Proliferating Cell Nuclear Antigen (PCNA) is a member of the sliding clamp family of DNA-replication accessory proteins. In most organisms PCNA is a homotrimer, in which its three subunits adopt a doughnut-shaped structure in a head-to-tail arrangement; this toroidal structure is extremely conserved in protozoa, humans, yeast and plants. The structure of PCNA is comprised by two α+β domains joined by an inter-domain connecting loop (IDCL). The inner face of the toroid has an array of basic residues positioned to provide favorable electrostatic interactions with the DNA-phosphate backbone.

Herein we report the x-ray structure analysis of the first crustacean recombinant PCNA (LvPCNA) and a model where PCNA interacts with viral DNA polymerase PIP-box as an approach toward structural understanding this feasible interaction. LvPCNA eluted in a complex of approximately 90 kDa, indicating that this protein assembles as a trimer in solution. Accordingly to this previous result the molecular replacement found a trimer in the asymmetric unit. LvPCNA had the cognate fold comprised by β-α-β5-α-β-β-β-IDCL-β-α-β5-α-β-β-β topology with pseudo symmetry within each monomer. The backbone cartoon shows the canonical structure and although the IDCL (residues 117–133) had poor electron density, the density was conclusive to include the coordinates of those residues in the final model. LvPCNA amino acid sequence is highly conserved among species and is structurally similar when compared with Drosophila PCNA, as it had a root mean square deviation (RSMD) of 0.5 Å for the α-carbon backbone. The central hole is highly positive charged as shown in Figure 3 and has a diameter of 30.5 Å, large enough to accommodate the double helical DNA and slide freely on it. A peptide sequence containing the WSSV DNA polymerase PIP box was modeled and docked into the crystallographic structure of shrimp PCNA, which is its natural host. However, this is a tight packing cavity as obtained by docking, where mostly hydrophobic interactions are leading the binding, the hydrophobic cavity is represented in a surface image where the PIP-box peptide is positioned and drawn as sticks. This pocket comes mainly from the IDCL (G127, P129, T131), central loop (S43, H44, V45, L47) and from C-terminus (F250, L251, A252, P253, I255) residues. The results from docking suggest that WSSV polymerase has the capacity of binding the LvPCNA in the same way that most PCNA binding proteins do.

>[3x]MFEARLVQGSLLKKVLEAIKDLLNEASWDCADSGIQLQAMDNSHVSLVSLNLRAKGFDKYRCDRNLIMGMNLTSMSKILKCAANDDIITMKAQDNADTVTFMFESPNQEKVSDYEMKLMNLDQEHLGIPETDYACVIKLPSGEFARICRDLSQFGESIVIACTKEGVKFSAAGDIGTANIKLAQTSSVDKEEEAVVIEMQEPVTLTFACRYLNMFTKATPLSPQVSLSMSPDVPLVVEYAIGEIGHIRYFLAPKIEDEDS> GSHMAKHEQILVLDPPSDLKFKGPFTDVVTTNLKLQNPSDRKVCFKVKTTAPRRYCVRPNSGVIDPGSIVTVSVMLQPFDY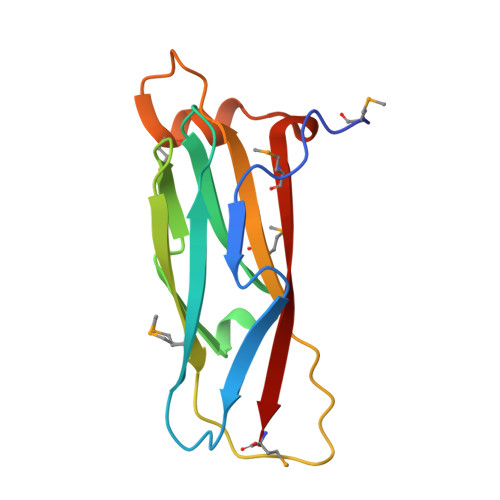DPNEKSKHKFMVQTIFAPPNISDMEAVWKEAKPDELMDSKLRCVFEM>MFGYFYNSSFRRYATLMGDLFSNIQIKRQLESGDKFIRVPITYASKEHFMMKLNKWTSINSQEDVAKVETILPRINLHLVDFSYNAPFKTNILNQNLLQKGATSVVSQYNPSPIKMIYELSIFTRYEDDMFQIVEQILPYFQPHFNTTMYEQFGNDIPFKRDIKIVLMSAAIDEAIDGDNLSRRRIEWSLTFEVNGWMYPPVDDAEGLIRTTYTDFHANTRDLPDGEGVFESVDSEVVPRDIDPEDWDGTVKQTFTSNVNRPTPPEPPGPRT[6x];>[6x]MTLLSPGIELKETTVQSTVVNNSTGTAALAGKFQWGPAFQIKQVTNEVDLVNTFGQPTAETADYFMSAMNFLQYGNDLRVVRAVDRDTAKNSSPIAGNIEYTISTPGSNYAVGDKITVKYVSDDIETEGKITEVDADGKIKKINIPTAKIIAKAKEVGEYPTLGSNWTAEISSSSSGLAAVITLGKIITDSGILLAEIENAEAAMTAVDFQANLKKYGIPGVVALYPGELGDKIEIEIVSKADYAKGASALLPIYPGGGTRASTAKAVFGYGPQTDSQYAIIVRRNDAIVQSVVLSTKRGGKDIYDSNIYIDDFFAKGGSEYIFATAQNWPEGFSGILTLSGGLSSNAEVTAGDLMEAWDFFADRESVDVQLFIAGSCAGESLETASTVQKHVVSIGDVRQDCLVLCSPPRETVVGIPVTRAVDNLVNWRTAAGSYTDNNFNISSTYAAIDGNYKYQYDKYNDVNRWVPLAADIAGLCARTDNVSQTWMSPAGYNRGQILNVIKLAIETPQAQRDRLYQEAINPVTGTGGDGYVLYGDKTATSVPSPFDRINVRRLFNMLKTNIGRSSKYRLFELNNAFTRSSFRTETAQYLQGNKALGGIYEYRVVCDTTNNTPSVIDRNEFVATFYIQPARSIN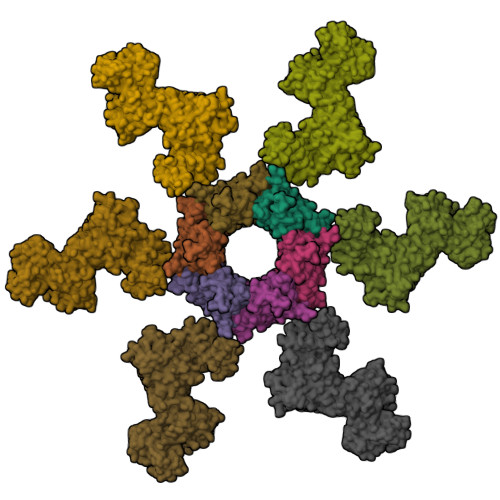YITLNFVATATGADFDELTGLAG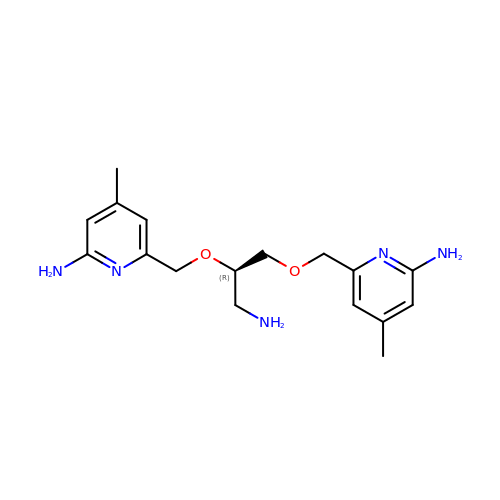6,6'-{[(2R)-3-aminopropane-1,2-diyl]bis(oxymethanediyl)}bis(4-methylpyridin-2-amine) | C17 H25 N5 O2 | FVCUZJIKIIWHJD-OAHLLOKOSA-N>[5x]MASTVSNTSKLEKPVSLIWGCELNEQNKTFEFKVEDDEEKCEHQLALRTVCLGDKAKDEFHIVEIVTQEEGAEKSVPIATLKPSILPMATMVGIELTPPVTFRLKAGSG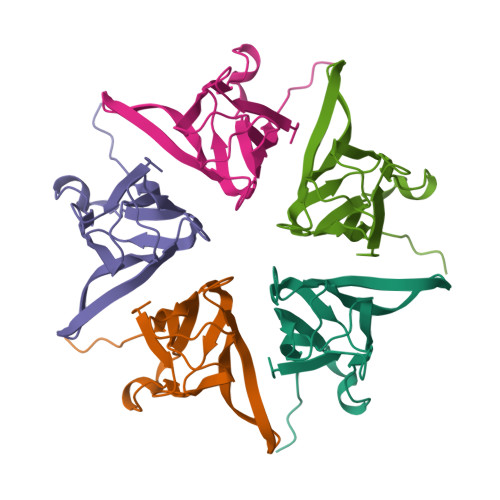PLYISGQHVAMEEDYSWAEEEDEGEAEGEEEEEEEEDQESPPKAVKRPAATKKAGQAKKKLDKEDESSEEDSPTKKGKGAGRGRKPAAKK>[3x]GSHMKNSVSVDLPGEMKVLVSKEKNKDGKYDLIATVDKLELKGTSDKNNGSGVLEGVKADKSKVKLTISDDLGQTTLEVFKEDGKTLVSKKVTSKDKSSTEEKFNEKGELSEKKITRADKSSTEEKFNEKGELSEKKITRADKSSTEEKFNEKGELSEKKI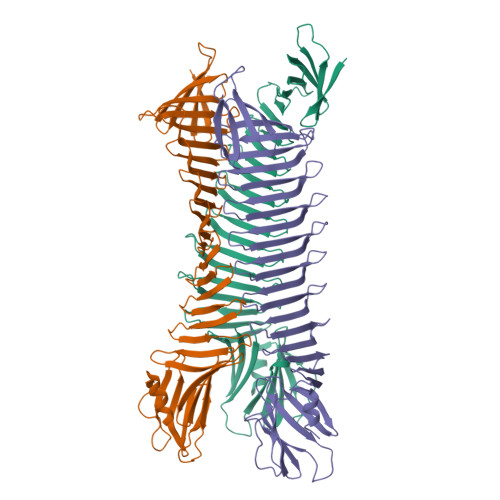TRADKSSTEEKFNEKGELSEKKITRADKSSTEEKFNEKGELSEKKITRADKSSTEEKFNEKGEVSEKIITRADGTRLEYTGIKSDGSGKAKEVLKGYVLEGTLTAEKTTLVVKEGTVTLSKNISKSGEVSVELNDTDSSAATKKTAAWNSGTSTLTITVNSKKTKDLVFTKENTITVQQYDSNGTKLEGSAVEITKLDEIKNALK>[2x]MTMEKGMSSGEGLPSRSSQVSAGKITAKELETKQSYKEKRGGFVLVHAGAGYHSESK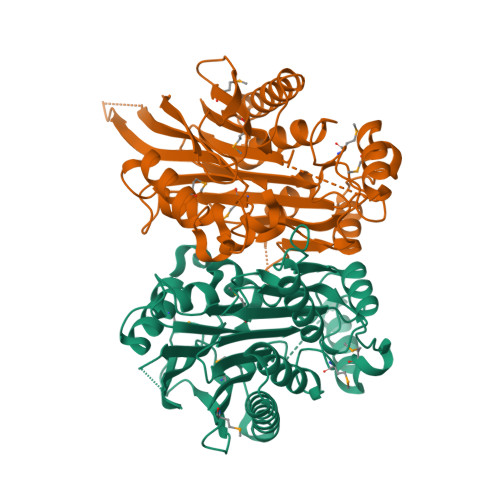AKEYKHVCKRACQKAIEKLQAGALATDAVTAALVELEDSPFTNAGMGSNLNLLGEIECDASIMDGKSLNFGAVGALSGIKNPVSVANRLLCEGQKGKLSAGRIPPCFLVGEGAYRWAVDHGIPSCPPNIMTTRFSLAAFKRNKRKLELAERVDTDFMQLKKRRQSSEKENDSGTLDTVGAVVVDHEGNVAAAVSSGGLALKHPGRVGQAALYGCGCWAENTGAHNPYSTAVSTSGCGEHLVRTILARECSHALQAEDAHQALLETMQNKFISSPFLASEDGVLGGVIVLRSCRCSAEPDSSQNKQTLLVEFLWSHTTESMCVGYMSAQDGKAKTHISRLPPGAVAGQSVAIEGGVCRLESPVN>[2x]QSLGQVKGHATFVKSMTTEMYQEQQNHSLAYNQRLASQNRIVDPFLAEGYEVNYQVSDDPDAV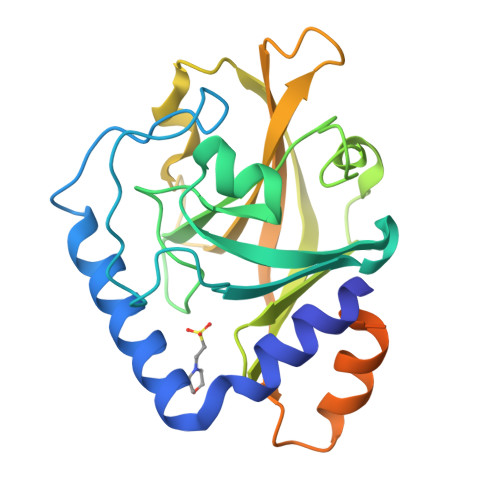YGYLSIPSLEIMEPVYLGADYHHLGMGLAHVDGTPLPLDGTGIRSVIAGHRAEPSHVFFRHLDQLKVGDALYYDNGQEIVEYQMMDTEIILPSEWEKLESVSSKNIMTLITCDPIPTFNKRLLVNFERVAVYQKSDPQTAAVARVAFTKEGQSVSRVATSQWLYRGLVVLAFLGILFVLWKLARLLRGK>MLEDLKRQVLEANLALPKHNLVTLTWGNVSAVDRERGVFVIKPSGVDYSIMTADDMVVVSIETGEVVEGAKKPSSDTPTHRLLYQAFPSIGGIVHTHSRHATIWAQAGQSIPATGTTHANYFYGTIPCTRKMTDAEINGEYEWE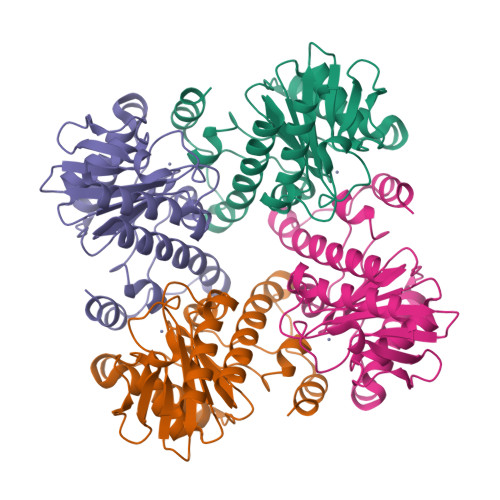TGNVIVETFEKQGIDAAQMPGVLVHSHGPFAWGKNAEDAVHNAIVLEEVAYMGIFCRQLAPQLPDMQQTLLNKHYLRKHGAKAYYGQ[6x]> MVARVQTAEEIRDEGNAAVKDQDYIKADELYTEALQLTTDEDKALRPVLYRNRAMARLKRDDFEGAQSDCTKALEFDGADVKALFRRSLAREQLGNVGPAFQDAKEALRLSPNDKGIVEVLQRLVKANNDKIKQTTSLANKVTDMEKLAFRGEAKDTEQKMTALNNLLVLCRESESGATGVWNQGALVPFVLNLINDASENEEVTVTAIRILDETIKNSVRCMKFLAMHDPDGPKSVRFVCRLMCKKSTKDFVDATGILVQRVFNAMAKMDRQKEMKPDPEVAEANKIWIIRVLLELQEMLQDPKVGAVQRETCIDLFLKNLMHMDGGIPRGWSWKFVEERGLLALLDVASQIPELCEYPVSAETRQHVAICLQRLEEDMVFDTKRTIFKEKVDMFFNALISRCTNDDEGHKYRIKLSCFLITMLQGPVDIGINLITNDQLTPIMLEMAASQDHLMQGIAAELIVATVSKHERAINMLKVGIPVLRALYDSEDPTVKVRALVGLCKIGAAGGDDISKATMKEEAVISLAKTCKKFLLETEKYSVDIRRYACEGLSYLSLDADVKEWIVDDSLLLKALVLLAKKAGALCVYTLATIYANLSNAFEKPKVDEEMVKLAQFAKHHVPETHPKDTEEYVEKRVRALVEEGAVPACVAVSKTESKNALELIARSLLAFAEYEDLRGRIIAEGGTVLCLRLTKEASGEGKIKAGHAIAKLGAKADPMISFPGQRAYEVVKPLCDLLHPDVEGKANYDSLLTLTNLASVSDSIRGRILKEKAIPKIEEFWFMTDHEHLRAAAAELLLNLLFFEKFYEETVAPGTDRLKLWVLYSAEVEEERLSRASAAGFAILTEDENACARIMDEIKSWPEVFKDIAMHEDAETQRRGLMGIANIMHSSNKLCSEIVSSEVFRVLVAVTKLGTINQERAGSTEQAKRGLEAAEKFGLIKATDREIYERENQMSTIQE

A major player in this process is the UCS (UNC-45/Cro1/She4p) protein UNC-45, a myosin chaperone critical for the assembly of thick filaments. Specifically, UNC-45 was shown to promote the folding of the motor domain of myosin molecules. In this process, UNC-45 acts as a co-chaperone together with the general chaperones Hsp70 and Hsp908,11,12.

While extensive crystallization trials of the UCS domain containing various KR mutations were not successful, we succeeded in crystallizing the wild-type UNC-45 protein in a crystal form, capturing the UCS domain in a distinct state. The corresponding structure of UNC-45717 (the number reflects the shortened crystallographic c-axis, when compared to the previously reported form, UNC-4581511) was determined at 3.8 Å resolution and exhibited a similar domain organization as UNC-45815: the chaperone adopts a V-shaped structure with the myosin-binding UCS domain opposing the core region constituted by the TPR, central, and neck domains. Like UNC-45815, the UNC-45717 molecule formed protein filaments in the crystal lattice using the same 4-helix interface to connect molecules. However, a pronounced structural change was seen in the UCS domain, a right-handed superhelix that was bent to different degrees reflecting two distinct conformational states. Structural alignment of the two states revealed a bipartite organization of the UCS domain. Its N-terminal (ARM repeats 10–12) and C-terminal (ARM repeats 14–17) halves are connected by the irregular ARM repeat 13, the hinge of the domain. The disrupted interfaces between ARM repeats 12/13 and 13/14 appear to provide the conformational flexibility to allow for a 15° rotation of the C-terminal portion, a gross rearrangement resulting in a 10 Å shift of the C-terminal ARM repeat. Although the N-terminal UCS half is held in position by the underlying central domain, B-factor values increase abruptly from ARM repeat 14, the first segment of the C-terminal UCS subdomain. Together, the crystallographic data underline the structural flexibility of the UCS domain, which can adopt discrete conformations. Strikingly, mapping the KRcanyon mutations on the structure showed that the corresponding lysine residues cluster in a well-defined region of the UCS domain, contributing directly to the interface of the N-terminal and C-terminal subdomains.> MAKQKYSEEVLDELRVDLQRRFNYAQGYVDMAVKGYAREAWEYFYGNLPAPVTAGSSSWVDRTVWESVNGTLQDIINVFCSGDEAVTFVADNQQDSDAADVATKLVNQILLRDNPGYNIISSAAQECLVTRNSFIKYYWDEQTSTQTEEAEGVPPEALAAYVQGLEAGGLKNLEVFTEENEDGTVDVKVTYEQTVKRVKVEYVPSEQIFVDEHATSFADAQYFCHRVRRSKEDLVAMGFPKDEIEAFNDWTDTMDTTQSTVAWSRTDWRQDIDADIGTDTEDIASMVWVYEHYIRTGVLDKNKESKLYQVIQAGEHILHTEEVTHIPFVTFCPYPIPGSFYGQSVYDITKDIQDLRTALVRGYIDNVNNANYGRYKALVGAYDRRSLLDNRPGGVVEMERQDAIDLFPYHNLPQGIDGLLGMSEELKETRTGVTKLGMGINPDVFKNDNAYATVGLMMNAAQNRLRMVCRNIAHNGMVELMRGIYNLIRENGEVPIEVQTPRGMIQVNPKQLPARHNLQVVVAISPNEKAERAQKLISLKQLIAADAQLAPLFGLEQDRYMTAQIFELMGIKDTHKYLLPLEQYQPPEPSPMEILQLEMTKAQVENVQASSQKMIADAFDQRERTTFEQQKAADELSLRQEELQFKQENAADAMTLENRKEDNNATLEQAKHKLALMQQQVRQYESVLKELQMVMSHQVDQEKIVQQARVQDKTLELQKKEANVTKKEQQASLKDSRIPGK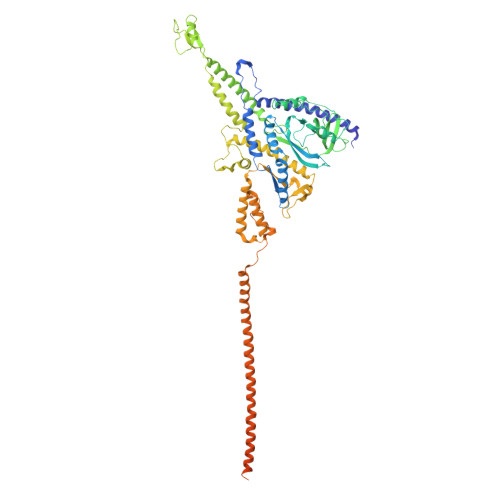RLGSKK>MAKGKSEVVEQNHTLILGWSDKLGSLLNQLAIANESLGGGTIAVMAERDKEDMELDIGKMEFDFKGTSVICRSGSPLILADLKKVSVSKARTIIVLAEDGNADQSDARALRTVLSLTGVKEGLRGHIVVEMSDLDNEVLVKLVGGDLVETVVAHDVIGRLMIQCARQPGLAQIWEDILGFENCEFYIKRWPQLDGMLFEDVLISFPAAIPCGIKVASYGGKIILNPDDSYVLQEGDEVLVIAEDDDTYAPAPLPMVRRGSLPKDFVYPKSPERILFCGWRRDMEDMITVLDASLAPDSELWMFNDVPEKEREKKLIDGGLDISRLENISLVNREGNAVIRRHLESLPLESFDSILILADESVEDSAIQADSRSLATLLLIRDIQARRLPYVAMASQTQGGNFSKGSWIGEMKQASDKTVIISEILDPRTKNLLSMSKISDYVLSNELVSMALAMVAEDRQINDVLEELFAEEGNEMHIRQADIYLREGEEMSFYEIMLRARQRREILIGYRLANAERAVINPPAKTGRRKWSLKDVFVVITEKEGSRSHHHHHH[4x]

Two DMI1 homologs, named POLLUX and CASTOR, were identified in L. japonicus and both of them are required to initiate symbiosis. To address these fundamental issues that define the primary function of these channels and their role in the symbiotic process, we performed functional characterization of the LjCASTOR channel and demonstrate that it functions as a Ca2+-regulated Ca2+ channel rather than as a K+ channel as previously proposed. We also determined the high-resolution crystal structure of the ligand-binding soluble domain of LjCASTOR and reveal that the entire soluble domain consists of two tandem RCK domains that assemble into a tetrameric gating ring where Ca2+ can bind and regulate the channel. Our high-resolution structure reveals multiple Ca2+-binding sites in the RCK gating ring and provides structural insights into Ca2+-regulated gating of CASTOR.

To reveal if Ca2+ binding induces a similar conformational change in CASTOR, we also crystallized the apo form of CASTOR gating ring with the presence of 1 mM ethylene glycol-bis(β-aminoethyl ether)-N,N,N′,N′-tetraacetic acid (EGTA). Compared to the Ca2+-bound form, CASTOR gating ring is biochemically less stable in the absence of Ca2+ as demonstrated by the broader and less symmetrical protein elution peak on a gel-filtration column. The obtained crystals diffracted to a much lower resolution and the final structure was determined to 3.3 Å. The crystal has a space group of P 21 and contains four subunits per asymmetric unit; the four subunits exhibit slight conformational heterogeneity among them and form an asymmetrical gating ring. In comparison to the Ca2+-bound state, the structural change between apo and Ca2+-bound subunits mainly involves rigid body movement of the N-lobe of RCK1, causing alterations in relative orientations between the subdomains. In the Ca2+-bound state, the N-lobe of RCK1 is tightened to the rest of the protein via two Ca2+-mediated interactions at cluster I and cluster II sites, respectively. Both interactions are missing in the apo state and consequently the RCK1 N-lobe has more freedom to undergo rigid body movement: at cluster I site, the RCK1 N-lobe slides apart from the RCK2 N-lobe; at the cluster II site, the RCK1 N-lobe swings away from the C-terminal subdomain, resulting in a slightly enlarged cleft between the two. In the context of gating ring, however, there is no significant change in the ring size of CASTOR with or without Ca2+. The two diagonal distances of the asymmetrical apo ring (between the Cα of Thr 323) are about 61 and 66 Å, respectively, whereas the equivalent distance is 62 Å in the symmetrical Ca2+-bound gating ring.> GPGQKIGILGAMREEITPILELFGVDFEEIPLGGNVFHKGVYHNKEIIVAYSKIGKVHSTLTTTSMILAFGVQKVLFSGVAGSLVKDLKINDLLVATQLVQHDVDLSAFDHPLGFIPESAIFIETSGSLNALAK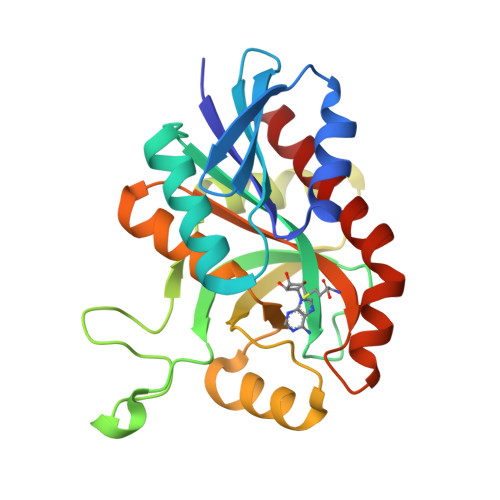KIANEQHIALKEGVIASGDQFVHSKERKEFLVSEFKASAVEMEGASVAFVCQKFGVPCCVLRSISNNADEKAGMSFDEFLEKSAHTSAKFLKSMVDEL> MALTQSVGGDSSADRLFPPQWICCDIRYLDVSILGKFAVVMADPPWDIHMELPYGTLTDDEMRRLNIPVLQDDGFLFLWVTGRAMELGRECLNLWGYERVDEIIWVKTN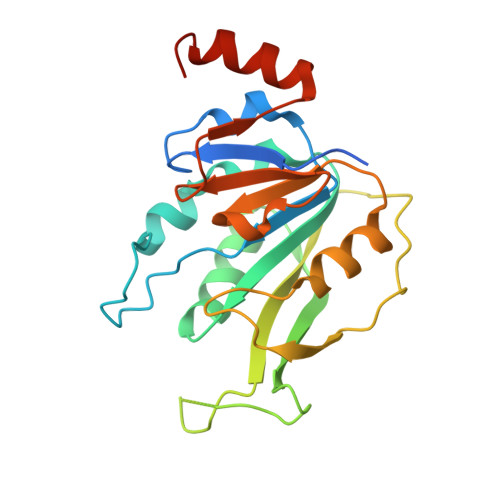QLQRIIRTGRTGHWLNHGKEHCLVGVKGNPQGFNQGLDCDVIVAEVRSTSHKPDEIYGMIERLSPGTRKIELFGRPHNVQPNWITLGNQLDGIHLLDPDVVARFKQRYPDGIISKPKNL> MKTEWPELVGKSVEEAKKVILQDKPAAQI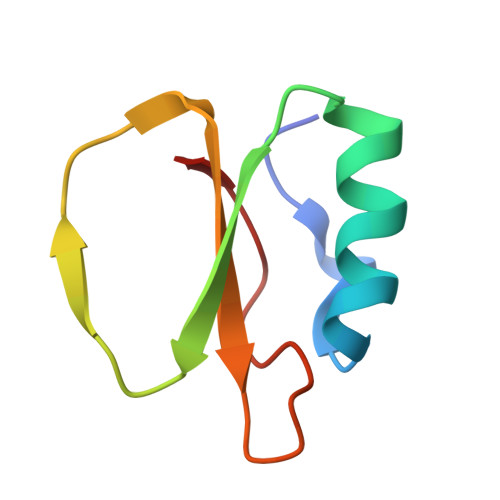IVLPVGTIVTRSYRIDRVRLFVDRLDNIAQVPRVG> MKREAIHNFFVANQIIKSTADMAIFDKVPATAIYEVMQVRQGIPLFFEAHLERFVMSASLVGTRIPKKEAEILHNIADLVEKNKCDHGNVKLVSALMNEKEIFLAYFIPAEFLDSKARLEGVHTILFSGERICPNIKTIKGSFREQVKAVRESSNAYEALLVNESGHITEGSRSNVFFMGKDNKLYTSPAGSVLKGVTRTHVMQICSRLGLEVLEKTVHTRNLADIQGAFITGTTVDVTPVRSIGNTQLDSPNIPLIRKIVAEYEKKIAGYVSKRLKRARKVYVND

Here, we describe a monomeric PLP-dependent fold type IV transaminase found in a marine aromatic-compound-degrading sulfate-reducing bacterium Desulfobacula toluolica Tol2. To the best of our knowledge, this is the first active monomeric PLP-dependent enzyme among the known fold type I and IV transaminases. The new monomeric transaminase (DtolTA) is stereoselective and active toward D-alanine and (R)-phenylethylamine. The results show that the active site of the transaminase, formed by a single subunit, is active in PLP-catalyzed deamination but is insufficient for double-substrate transamination.

Two crystal structures of DtolTA were obtained, one at 2.6 Å (low resolution, space group F4132) and another at 1.8 Å (high resolution, space groups P212121). As part of the subunit had no electron density in the high-resolution structure, the low-resolution structure was used to describe the overall structure, while the high-resolution structure was used to describe the active site of DtolTA. A total of 30 residues at the N-terminus and 9 residues at the C-terminus had no electron density in DtolTA (high resolution), while in DtolTA (low resolution), the entire polypeptide chain was clearly visible. According to the crystallographic contacts, DtolTA is a monomer, and no functional dimer similar to bsDATA was found in the crystal cell based on contact analysis. Similarly to the known transaminases of PLP fold type IV, the subunit of DtolTA consists of two α/β domains: a small domain (residues 1–107) and a large domain (residues 122–286) connected by the interdomain loop (residues 108–121). The DtolTA monomer is distinguished by the O-pocket loop (residues 97–100), which is significantly shorter than that in bsDAAT (residues 92–110), the C-terminal α-helix (residues 256–286), which is approximately twice as large as that in bsDATA (residues 263–277), and, finally, by the unique position of the O-pocket α-helix (residues 22–27). Two regions (regions 1 and 2) important for dimerization in classical transaminases were identified and analyzed. In DtolTA, region 1 (C and pink rectangle in Figure 5) was shorter than in other transaminases and included an α-helix (residues 22–27), so that the residues of region 1 did not protrude from the subunits as in homologous transaminases. In addition, in DtolTA, the position of α-helix 22–27 was reinforced by the salt bridge Asp26–Arg3. This salt bridge also positioned the N-terminus directly at the dimer interface, preventing dimer formation. Other structural elements involved in the formation of the dimer interface in bsDATA, eBCAT, and R-ATA have the same spatial arrangement as in DtolTA. It is worth noting that the long C-terminal α-helix of DtolTA does not affect the formation of the classical dimer, but appears to contribute to the stabilization of the monomer via hydrogen bonds between its residues and residues of the small and large domains: E265-R40, Y271-E48, and R275-nitrogen atom of the main chain of F47.> GPLGHMSIFEKDLMAYFDENLNRNWRGREHWKVRNFKKANLVNKESDLLEETRTTIGDTTDKNTTDDKSMDTKKKHKQKKVLEIDFFKTDD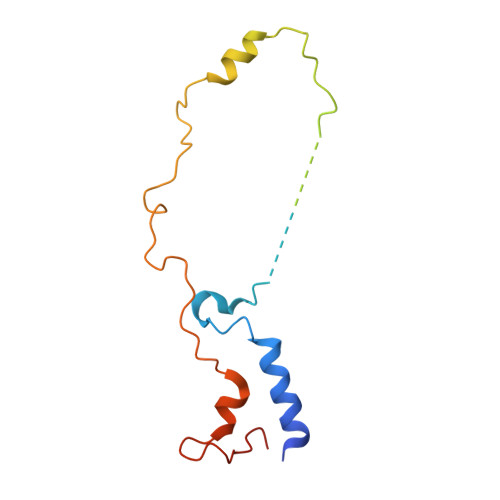SFEDKVFASKGRTKIDMPIKNRKNDTHYLLPDDFHFSTDRITRLFIKPGQKMSLFSHRKHT>MNKAQIEIYYCRQCNWMLRSAWLSQELLHTFSEEIEYVALHPDTGGRFEIFCNGVQIWERKQEGGFPEAKVLKQRVRDLIDPERDLGHVDRPSSTQS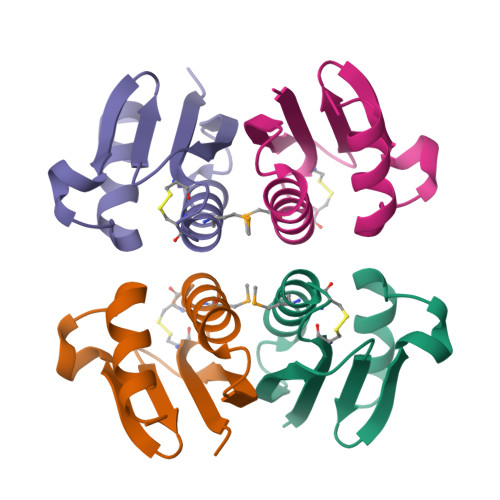LEHHHHHH[4x]> GSGSDEKICAIYPHLKDSYWLSVNYGMVSEAEKQGVNLRVLEAGGYPNKSRQEQQLALCTQWGANAIILGTVDPHAYEHNLKSWVGNTPVFATVNQLDLDEEQSTLLKGEVGVDWYWMGYEAGKYLAERHPKGSGKTNIALLLGPRTRGGTKPVTTGFYEAIKNSDIHIVDSFWADNDKE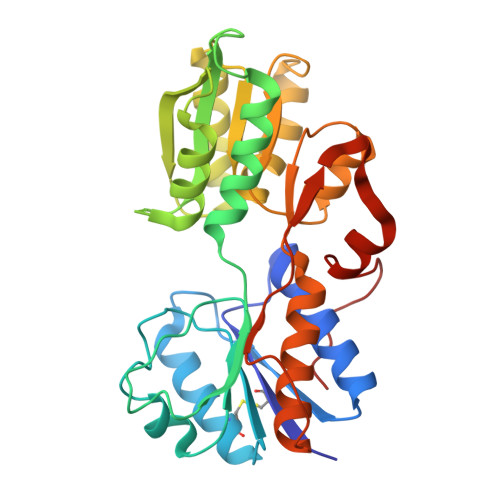LQRNLVQRVIDMGNIDYIVGSAVAIEAAISELRSADKTHDIGLVSVYLSHGVYRGLLRNKVLFAPTDKMVQQGRLSVMQAAHYLRHQPYEKQASPIIKPLTPKTLHDDTIEESLSPSEYRPTFS> GPTATAPGGLSAKAPAMTPLMLDTSSRKLVAWDGTTDGAAVGILAVAADQTSTTLTFYKSGTFRYEDVL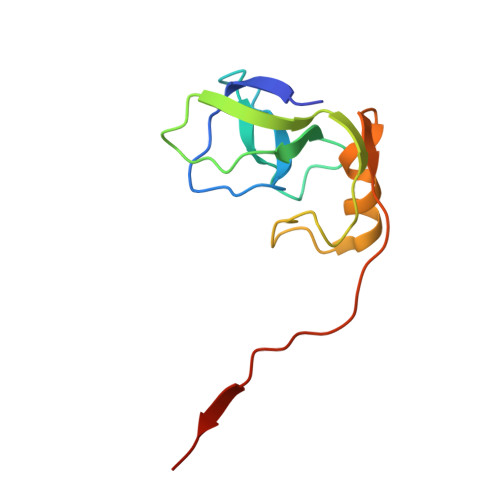WPEAASDETKKRTAFAGTAISIVGSGSPKRKRKRKRKREG> MAEESRGQRGSGYGLGLSTRTQVTGYQFLARRTAMALTRWRVRMEIEPGRRQTLAVVASVSAALVICLGALLWSFISPSGQLNESPIIADRDSGA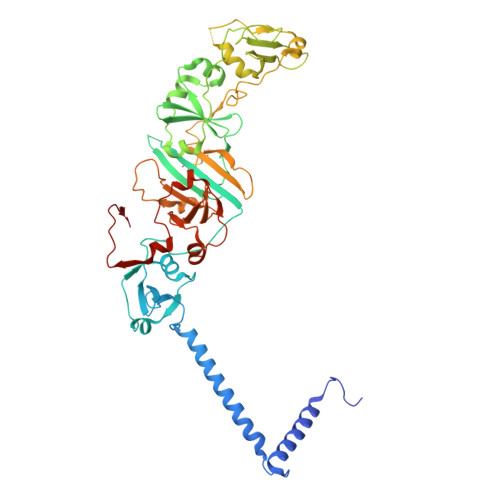LYVRVGDRLYPALNLASARLITGRPDNPHLVRSSQIATMPRGPLVGIPGAPSSFSPKSPPASSWLVCDTVATSSSIGSLQGVTVTVIDGTPDLTGHRQILSGSDAVVLRYGGDAWVIREGRRSRIEPTNRAVLLPLGLTPEQVSQARPMSRALFDALPVGPELLVPEVPNAGGPATFPGAPGPIGTVIVTPQISGPQQYSLVLGDGVQTLPPLVAQILQNAGSAGNTKPLTVEPSTLAKMPVVNRLDLSAYPDNPLEVVDIREHPSTCWWWERTAGENRARVRVVSGPTIPVAATEMNKVVSLVKADTSGRQADQVYFGPDHANFVAVTGNNPGAQTSESLWWVTDAGARFGVEDSKEARDALGLTLTPSLAPWVALRLLPQGPTLSRADALVEHDTLPMDMTPAELVVPK>[2x]GSAMGSASTS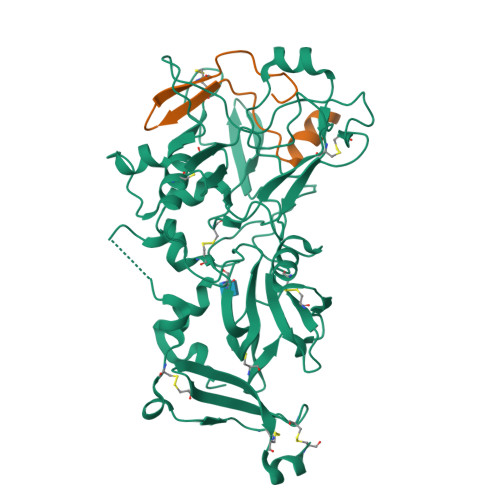GNPFQANVEMKTFMERFNLTHHHQSGIYVDLGQDKEVDGTLYREPAGLCPIWGKHIELQQPDRPPYRNNFLEDVPTEKEYKQSGNPLPGGFNLNFVTPSGQRISPFPMELLEKNSNIKASTDLGRCAEFAFKTVAMDKNNKATKYRYPFVYDSKKRLCHILYVSMQLMEGKKYCSVKGEPPDLTWYCFKPRKSVTENHHLIYGSAYVGENPDAFISKCPNQALRGYRFGVWKKGRCLDYTELTDTVIERVESKAQCWVKTFENDGVASDQPHTYPLTSQASWNDWWPLHQSDQPHSGGVGRNYGFYYVDTTGEGKCALSDQVPDCLVSDSAAVSYTAAGSLSEETPNFIIPSNPSVTPPTPETALQCTADKFPDSFGACDVQACKRQKTSCVGGQIQSTSVDCTADEQNECGSNTAAALVPR;>DIVQHMEDIGGAPPVSCVTNEILGVTCAPQAIAKATX[2x]> MIEAPDVKPWLFLIKPYEGESLSHFLGRFRRANHLSASGLGTLAGIGA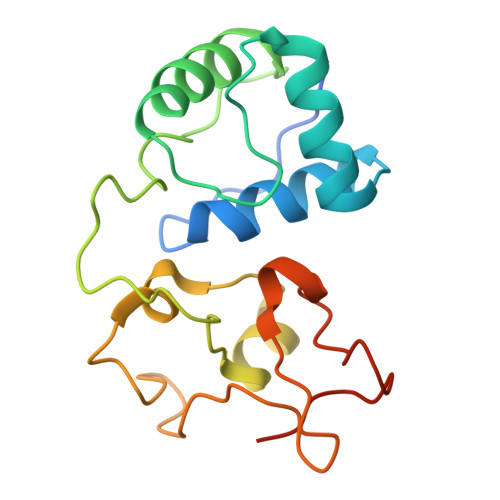IVARWERFHFNPRPSQQELEAIASVVEVDAQRLAQMLPPAGVGMQHEPIRLCGACYAESPCHRIEWQYKSVWKCDRHQLKILAKCPNCQAPFKMPALWEDGCCHRCRMPFAEMAKLQKV pmcTransmembrane β-barrel (TMB) nanopores formed by a circularly closed single β-sheet provide rigid scaffolds for the transport of molecules across cellular and organelle membranes. Encouraged by the success in designing these narrow TMBs, we reasoned that de novo protein design should provide a general approach to creating robust β-barrel nanopore scaffolds for a next generation of nanopore sensors. We set out to develop general methods to overcome these challenges and design stable monomeric channels with tunable pore shapes, sizes, and single-channel conductance. Our results demonstrate that it is possible to systematically design transmembrane β-barrels with conducting pores spanning a range of sizes and shapes.

To modulate the size of the pore, we increased the number of β-strands (10, 12, and 14 strands) while keeping the transmembrane span and the connectivity between β-strands (the shear number) constant. The first-generation backbones corresponding to these designs were assembled with the Rosetta BlueprintBDR application and had similar cylindrical shapes. Such cylindrical β-sheet configurations are strained as a result of repulsion between side chains packing the barrel lumen. Glycine kinks (glycine residues in extended positive-φ conformation) were introduced into the blueprint to relieve the strain and to bend the β-strands to form corners in the β-barrel cross section. In the water-accessible pore, networks of polar residues were designed around the canonical TMB folding motif Tyr-Gly-Asp/Glu to optimize strong local β-register–defining interactions while alternating with patches of hydrophobic and small, disorder-promoting residues (Gly, Ala, Ser). On the lipid-exposed surface, design calculations favored Ser and Thr in close proximity to a glycine kink where they could form a hydrogen bond to the β-strand backbone, effectively mimicking the backbone-water hydrogen bonds observed in strongly bent β-strands of water-soluble β-barrels. Although it is perhaps counterintuitive to expose hydroxyl groups to the lipid environment, we included a small number of these amino acids on the lipid-exposed surface instead of hydrophobic β-branched residues to further reduce the β-sheet propensity. As previously observed for eight-stranded TMBs, a delicate balance between the optimization of tertiary structure energy and negative design (introduction of locally frustrated residues) to disfavor premature β-strand formation before membrane insertion was critical for the expression of the larger TMB nanopores in E. coli inclusion bodies. Despite the inversion of the hydrophobic exterior and polar core compared with globular proteins and the almost entirely local nature of the side chain interactions, our approach enables TMB design with atomic level precision, as highlighted by the close agreement between the experimentally determined crystal and NMR structures and the corresponding design models.

>[4x]RTSPGTKPYVKVRWNTDNTVAVAFGAETDYKLAPYLKTGVATETEYNNSSLVKTGTEVKTAYRLGPNAALETVVRYNTDNTFGVEVAIEYRLEPDLSVAPGTRWNNSSLLAPYIKIKYKLGPDLDVVTTIAYNTDNTVGIETKVAYKTD> GNIYIS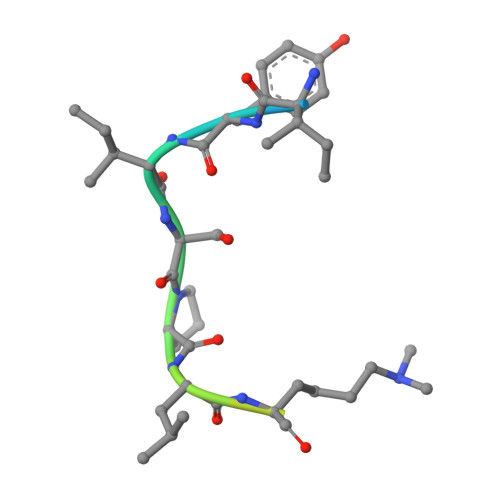PLKSPYKISEC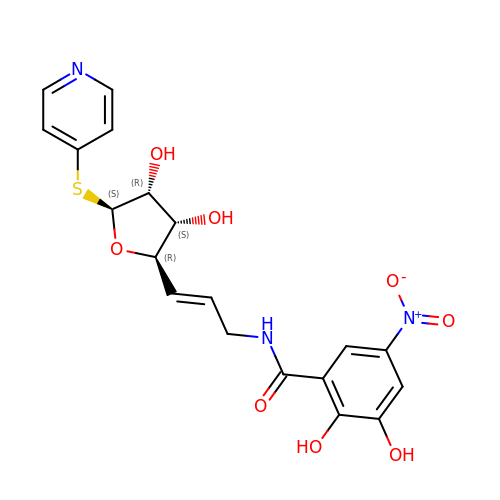N-[(E)-3-[(2R,3S,4R,5S)-3,4-dihydroxy-5-pyridin-4-ylsulfanyl-oxolan-2-yl]prop-2-enyl]-2,3-dihydroxy-5-nitro-benzamide | C19 H19 N3 O8 S | XRZIENNFYKGKSZ-GXSCOFJOSA-N>[2x]GSPRTVEEVFSDFRGRRAGLIKALSTDVQKFYHQCDPEKENLCLYGLPNETWEVNLPVEEVPPELPEPALGINFARDGMQEKDWISLVAVHSDSWL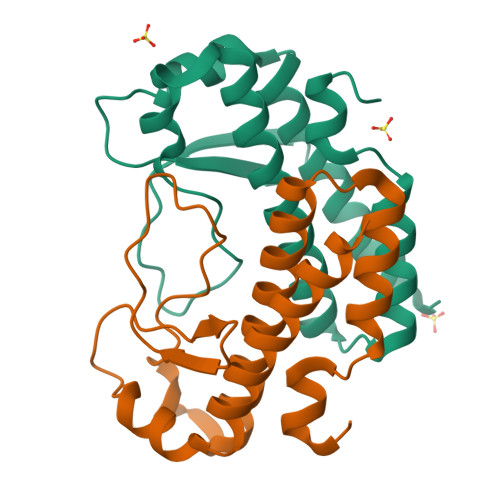ISVAFYFGARFGFGKNERKRLFQMINDLPTIFEVVTGNA>[2x]GPLGSMQYVGPYRLEKTLGKGQTGLVKLGIHCVTCQKVAIKIVNREKLSESVLMKVEREIAILKLIEHPHVLKLHDVYENKKYLYLVLEHVSGGELFDYLVKKGRLTPKEARKFFRQIISALDFCHSHSICHRDLKPENLLLDERNNIRIADFGMASLQVGDSLLETSCGSPHYACPEVIRGEKYDGRKADVWSCGVILFALLVGALPFDDDNLRQLLEKVKRGVFHMPHFIPPDCQSLLRGMIEVDAARRLTLEHIQKHIWYIGGKNEPEPEQPIPRKVQIRSLPSLEDIDPDVLDSMHSLGCFRDRNKLLQDLLSEEENQEKMIYFLLLDRKLEHHHHHH

The SAD (synapses of amphids defective) kinases, conserved across a wide range of species, play important roles in multiple phases of axonal development and function. Despite the diverse functions, the AMPK family members display similar structural organization, with an N-terminal kinase domain followed by a non-catalytic region containing an ubiquitin associated (UBA) domain and, in some cases, a kinase associated (KA1) domain. The C-terminal non-catalytic region of SAD kinases includes two short conserved regions, SCR1 and SCR2, which respectively contain the characteristic UBA and KA1 domains12731. In this study, structural and biochemical analyses of mouse SAD-A revealed a synergistic model for the autoinhibition of SAD activity by two separable elements, a newly identified autoinhibitory sequence (AIS) and the UBA domain.

To understand the autoinhibitory mechanisms, we first determined the crystal structure of mouse SAD-A fragment containing both kinase and UBA domains. This KD-UBA structure comprises a head-to-tail dimer per asymmetric unit, which is probably a crystallization artifact owing to its monomeric state in solution. The kinase domain of SAD-A folds into a canonical bilobed structure in which the N-lobe consists of a β-sheet and the prominent αC helix and the C-lobe is composed mainly of α-helices. A flexible linker connects the catalytic domain to the UBA domain of three-helix bundle. Distinctly, the SAD-A kinase adopts a third binding mode, mainly with the N-lobe of the kinase domain and weakly with the C-lobe. The KD–UBA interaction in SAD-A primarily involves two helices, α3 from the UBA domain and αC from the kinase domain, which buries ∼1,500 Å2 exposed surface area. Six conserved residues from the UBA domain pack against a hydrophobic patch at the C terminus of the prominent αC helix. Structural comparison reveals that the KD–UBA interaction in SAD-A brings helix αC into an orientation that is rotated outwards approximate 90° from that in the active kinases including AMPK ortholog Snf1 and the prototype PKA. The N-terminal portion of the partially disordered activation segment folds back into the active site, strictly preventing the formation of salt bridge(s) between Glu67 on helix αC and Lys49 on strand β3. Therefore, the distinct UBA binding mode and the inserted activation segment lead to a typically inactive (αC-out) kinase conformation, where the important Glu67 is 12.5 Å away from Lys49.>[2x]HHHHGSKTLPDKFLGTFKLERDENFDEYLKARGYGWIMRQVIKLAGVTKKFRNAASGKPDRYDMENLTTKKDTHHKDWALGEEFQDEALDSTQHKITFDLKDPNTLTETHIKVDDPTDVETYEYRRDGDYLVMKMSWKGVSTSRYYKKQ

Here we present the structure of a nemFABP, As-p18, from A. suum, a close relative of the large intestinal roundworm of humans, Ascaris lumbricoides. The nemFABPs as a subfamily of iLBPs therefore appear to be confined to nematodes, and are distinguished by being structurally distinct, secreted from cells by a conventional (secretory leader peptide-mediated) pathway, and may be associated with particular functions in nematode reproduction and development. We find that this protein, and probably all nemFABPs, has a fold similar to that of other iLBPs, but that it possesses two extended loops so far found definitively only in nemFABPs, with the largest of these loops being remote from the presumed portal of entry for ligands and the binding site itself. The NMR and X-ray-derived structures of As-p18 agree closely (RMSD = 0.46 Å) and exhibit features that characterize the FABP family, namely the β-clamshell structure comprising 10 antiparallel β-strands capped by a helix-turn-helix section.

Using a micro-focus beamline, a dataset was collected with diffraction observed to beyond 2.2 Å. Due to clear evidence of radiation damage, the data were processed and scaled to a maximum resolution of 2.3 Å. As-p18 crystalized with two near-identical copies of the protein in the asymmetric unit (coordinate RMSD 0.19 Å for all equivalent heavy atoms), but with incomplete electron density in the ligand-binding pockets. In the crystal structure of As-p18, the electron density associated with the co-purifying ligand was of insufficient resolution to determine its conformation unambiguously. The electron density within the binding pocket indicates that a single resident fatty acid molecule could be in a U-shaped conformation as observed for other FABPs, and sit with its charged head group either buried within the protein’s binding pocket, or pointing out towards the pocket’s opening. The head group buried orientation is the more likely given the precedence set by other FABPs and our NMR data. Since As- p18 predominantly co-purifies with vaccenate, we fitted this ligand into both copies of the protein in the asymmetric unit. In E. coli, these are principally 18:1 and for As-p18 almost exclusively vaccenate (cis-11-octadecenoate). In both the NMR- and X-ray-derived structures, the N-terminal residues Asp5-Phe7 form a 310- helical loop that is an extra secondary structure element characteristic of the subfamily IV in mammalian FABPs. The βB-βC loop is poorly defined in solution, consistent with the high crystallographic B factor values for this region, but there is limited evidence for flexibility from the 15N relaxation data.> ADFEVHMLNKGKDGAFVF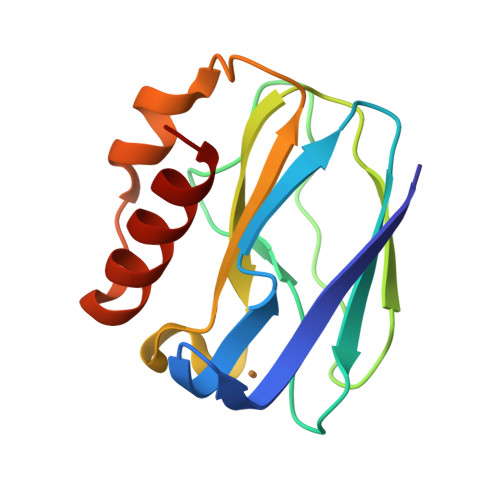EPASLKVAPGDTVTFIPKDKGHNVETIKGMIPDGAEAFKSKINENYKVTFTAPGVYGVKCTPHYGMGMVGVVQVGDAPANLEAVKGAKNPKKAQERLDAALAALGN>GPMEADGRYYSSKQPYVAPNDATASSYSKAPKGYGPIYTESMARHGSRGLSSYKYDALLMRMAETAARDGGFKSEAIKAEFVKNLSGITAANVENGYGMLTGQGAQQHYGIGERAYQRNRSLFDQAAADGGTIAYQSSGEARATESGENFEKGFNEASGGRLIGNVSAPTNPADSGNGKDFQKNPDTLYFHKVQNPDGTSKVPGTKAYDIANNYQNFVANDATIAGAEKTIGDNVDVKRASHDLLSQIFTEEFLAKLENGEYKWYNTTDGTKKGGKNCAPGADASKDPDACGEVSKKIKSEYDAAMDLYNLYIIAADMHNENTGDHTFAFDQYFQGAYADDARMFAWALDAEDFYEKGPSYAGQNETYSIAQPLLDDFLNTIDARVNGGSTVATFRFAHAETMMPFAALLGLPGSTQQAPASTTDVYTYGNNEWRGESVTPMAANVQWDVYARKGEDPATGQRYTPIVRMLYNENEVPFRSECTPVADGSTWYKLTELKSCLAADHKTLGQDARI[2x]

The multiple inositol polyphosphate phosphatases (MINPPs) constitute a distinct evolutionary group within clade 2 of the histidine phosphatase superfamily. To gain a wider understanding of the implications of these insertions on the properties of these enzymes, we carried out a crystal structure and mutagenic analysis of a representative member, BlMINPP, a moderately thermophilic, membrane-anchored extracellular enzyme. In keeping with previously reported crystal structures of HP2P family members, the structure of BlMINPP consists of two domains, an α/β-domain and an α-domain. The catalytic center of BlMINPP consists of the nucleophilic histidine (His-45), three arginine residues (Arg-44, Arg-48, and Arg-142), which coordinate the scissile phosphate during catalysis, and the amino acid triplet HAE (residues 339-401) where the glutamic acid residue acts as the presumed proton donor during catalysis.

To this end, crystals of the apoenzyme and of an inactive mutant in which the presumed catalytic proton donor Glu-401 was replaced by a glutamine (E401Q) were prepared, the latter in an attempt to trap the catalytic phosphohistidine intermediate. The structures of the apoenzyme and product complex were solved at 1.65 and 1.71 Å resolution, respectively, whereas a data set collected at 2.40 Å resolution from a crystal of the inactive E401Q mutant yielded a structure of the His-45 phosphohistidine derivative. Analysis of the resulting structures indicates that, unlike previously characterized HP2P, BlMINPP possesses an unusual inherent flexibility. In the apo-state the enzyme exists in an open conformation with many of the specificity pockets incompletely formed. On binding the substrate analog, the enzyme moves to a closed conformation where the full array of interactions with ligand are present. This movement is not limited to the active center, as is seen in E. coli AppA, but rather it propagates to a large region of the α-domain, which we will refer to as the molecular “lid,” which rotates on binding of substrate toward the α/β-domain. The lid comprises the majority of the α-domain residues, excluding only the residues of helices Ala-222–Ile-231 and Ala-337–Lys-357, which line one side of the active site cleft and the latter of which contributes residues to specificity pocket B. DynDom identified a maximum rotational movement of the lid of 18.1° upon ligand binding, corresponding to 82.3% closure of the moving domain. The α/β-domain and the remainder of the α-domain undergo only limited changes and are considered fixed (RMS deviation 0.55 Å).>MGKVIRSLNRFGKKVGNALTSNTAKKIYSTIGKAAERFAESEIGSAAIDGLVQGSVHSIITGESYGESVKQAVLLNVLGSGEEIPDPLSPGERGIQAKLKELEDEQRNELVRLKYNDKIKEKFGKELEEVYNFMNGEANAEIEDEKQFDILNKAVTSYNKILTEEDLQMRRLATALQKEIGERTHAETVMVKEYRDKIDALKNAIEVERDGMQEEAIQEIAGMTADVLEAASEEVPLIGAGMATAVATGRAIEGAYKLKKVINALSGIDLTHLRTPKIEPSVVSTILEYRAKEIPDNALAVSVLSKNRAIQENHKELMHIKNEILPRFKKAMDEEKEICGIEDKVIHPKVMMKFKIPRAQQPQIHVYSAPWDSDDVFFFHCISHHHANESFFLGFDLSIDLVHYEDLTAHWHALGAAQTAAGRTLTEAYREFLNLAISNAFGTQMHTRRLVRSKTVHPIYLGSLHYDISFSDLRGNAQRIVYDDELQMHILRGPIHFQRRAILGALKFGCKVLGDRLDVPLFLRNA[6x];>[3x]MDELGIPVYKRGFPEHLLRGYEFIIDVGTKIESVGGRHDVTKIPEMNAYDIKQESIRTALWYNPIRNDGFVLPRVLDITLRGYDERRAVVESTRHKSFHTNDQWVQWMMKDSMDAQPLKVGLDDQSRNVAHSLHNCVVKIDSKKADTMSYHVEPIEDASKGCLHTRTMMWNHLVRIETFHAAQEVAYTLKPTYDIVVHAERRDRSQPFRPGDQTLINFGRGQKVAMNHNSYDKMVEGLTHLVIRGKTPEVIRDDIASLDEICNRWIQSRHDPGEIKAYELCKILSTIGRKVLDREKEPEDEANLSIRFQEAIDNKFRQHDPERLKIFEHRNQRRDEDRFYILLMIAASDTFNTRVWWSNPYPCLRGTLIASETKLGDVYSMMRSWYDWSVRPTYTPYEKTREQEKYIYGRVNLFDFVAEPGIKIVHWEYRLNHSTREITYAQGNPCDLYPEDDDVIVTKFDDVAYGQMINEMINGGWNQEQFKMHKILKSEGNVL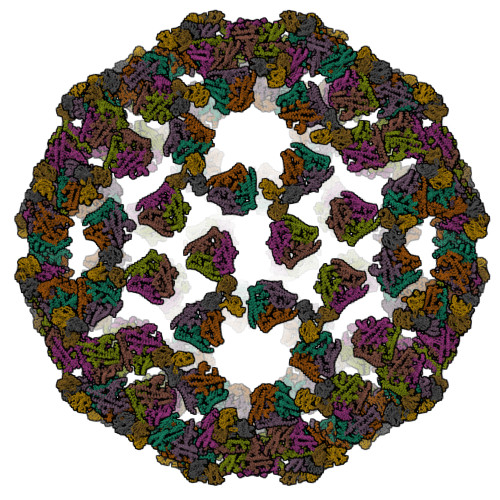TIDFEKDAKLTTNEGVTMPEYFNKWIIAPMFNAKLRIKHEEIAQRQSDDPMVKRTLSPITADPIELQRLTLARFYDIRPALRGQALSRQQAQSTYDEEISKQRDY> MSNMEKHL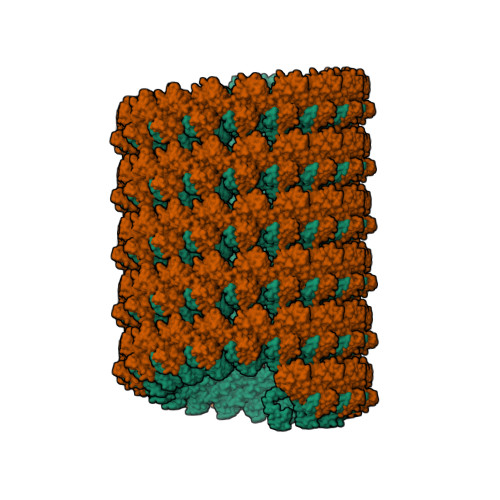FNLKFAAKELSRSAKKCDKEEKAEKAKIKKAIQKGNMEVARIHAENAIRQKNQAVNFLRMSARVDAVAARVQTAVTMGKVTKSMAGVVKSMDATLKTMNLEKISALMDKFEHQFETLDVQTQQMEDTVSSTTTLTTPQNQVDMLLQEMADEAGLDLNMELPQGQTGSVGTSVASAEQDELSQRLARLRDQV;> MLGSGFKAERLRVNLRLVINRLKLLEKKKTELAQKARKEIADYLAAGKDERARIRVEHIIREDYLVEAMEILELYCDLLLARFGLIQSMKELDSGLAESVSTLIWAAPRLQSEVAELKIVADQLCAKYSKEYGKLCRTNQIGTVNDRLMHKLSVEAPPKILVERYLIEIAKNYNVPYEPDSVVMAEAPPGVETDLIDVGFTDDVKKGGPGRGGSGGFTAPVGGPDGTVPMPMPMPMPSANTPFSYPLPKGPSDFNGLPMGTYQAFPNIHPPQIPATPPSYESVDDINADKNISSAQIVGPGPKPEASAKLPSRPADNYDNFVLPELPSVPDTLPTASAGASTSASEDIDFDDLSRRFEELKKKT> GAMVSGQIMHAVGEEGGHVKYVCKIENYDQSTQVTWYFGVRQL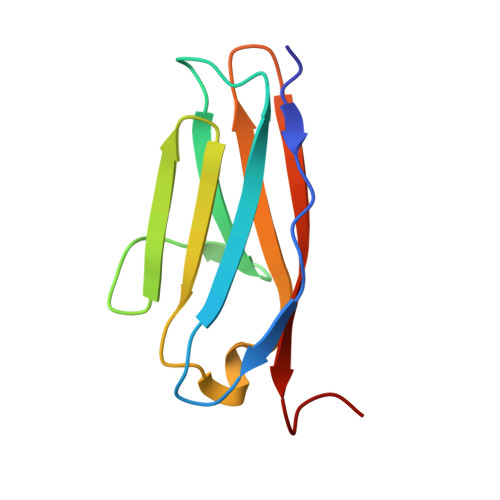ENSEKYEITYEDGVAILYVKDITKLDDGTYRCKVVNDYGEDSSYAELFVKGVRE> GSTGSPPGPPEDVTIDEITDTTAQLSWRPGADNHSPITMYVVQARTPFSVGWQAVSTVPEVIDGKTFTATVVGLNPWVEYEFRVVAANLIGIGEPSRPSENRRTEEALPEVTPANVSGGGGSKSELVITWETVPEELQNGGGFGYVVAFRPFGTISWMQAAVASPDASRYVFRNESLPPFSPYEVKVGVANNKGAGSFSPVTVVYSA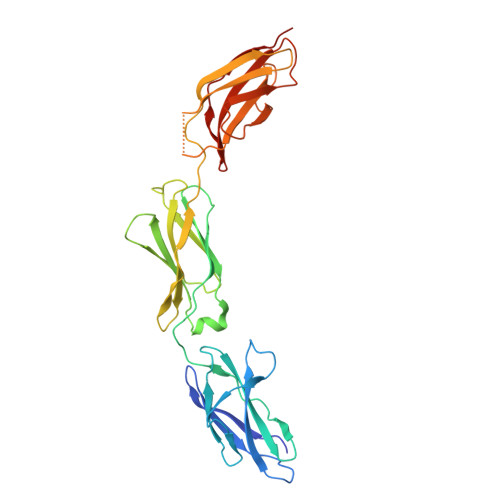EEEPTRAPITVLARSLSATDIEISWAPPRENQHKGRIQGYEVRCWRHDEKEENARKIRTVGNQTSAKVTNLQGNALYHLAVKAYNTAGTGPSSAMVNVTTKK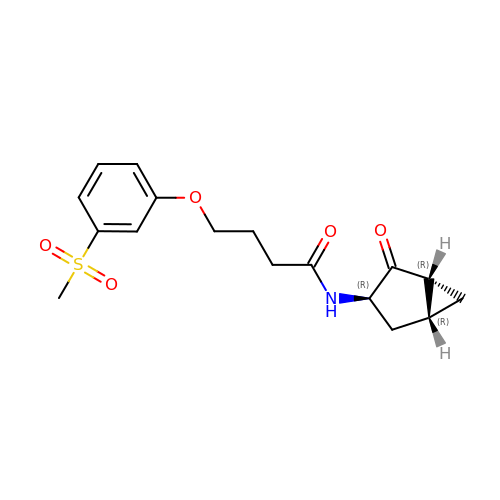4-[3-(methylsulfonyl)phenoxy]-N-[(1R,3R,5R)-2-oxobicyclo[3.1.0]hexan-3-yl]butanamide | C17 H21 N O5 S | MNLBJMNPVMBTLW-KCPJHIHWSA-N> AGACG;>CGTGGA[2x];> TCCGA;> CTACG;> TCCT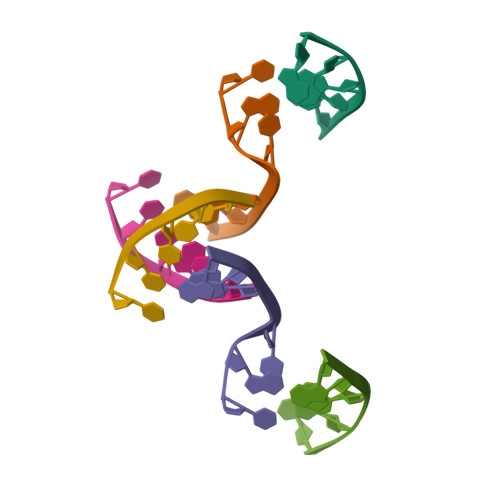C> MRASFLLTAGLATAAVGRAKSVPKKFPFKPENSKTTGTNAIPIVYGLSESQPNSVGGSWWSSSYITTTNNEQYVVLAHYLDNPVYTYFRASTLNLETNEYHQYVTVGSSTPNITTLDVSVGNNGIKSESEDNLSKLRSYSNHDNVTFDITYDATTGAVANGGAGTFQFGEGLTWEFGLPSAKTEGSLTVHGEKLAIDPAKSHT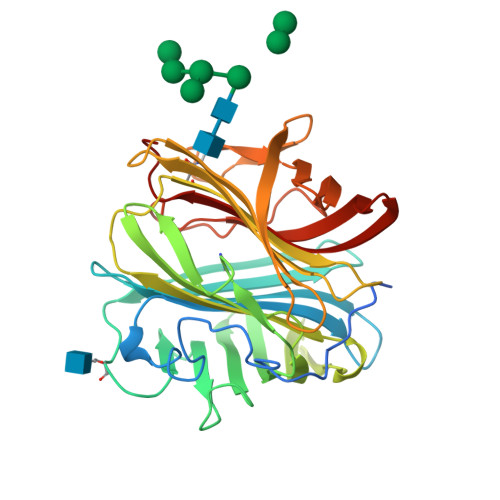WYDRQWGNTAAIPSNWTWFQLHIPSTEYKISAWIFSDPFRNTETRFATIRGANDETLVLPLEFTPIYKRTYESATGRVTYPLDWKLKISGFGDFKLSSYTEDQELVGEDALQTAYEGFITFSGNVHSKPVQGYGLVEIVYSTWDV>MASMSFGKFFNTAVSAWMSQEGPNSDIVLSSRIRLARNIVDFRFPTLFSSEEAKQIVALFERAFVHRPYGEAGRFELLKMSELQPIEKRVLVEKHLISPHLAEDSPFGACLLSENEEISIMINEEDHIRIQCLFPGLQLAEALEAASELDDWIEGHVNYAFDERLGYLTSCPTNVGTGLRASVMMHLPALVLTQQINRIIPAINQLGLVVRGTYGEGSEALGNIFQISNQITLGKSEEDIVADLHTIVEQLIAQERAARQALVKTLGIQLEDKVFRSYGILANCRVIDSKEAAQCLSDVRLGIDLGYIKNVSRNILNELMILTQPGFLQQYAGGVLRPEERDVRRAALIRERLR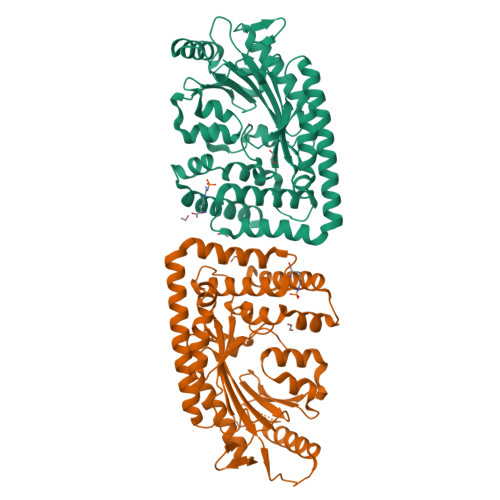METRLEHHHHHH[2x]> MVIRVLFRPVSLIPVNNSSTPQSQGPISRRLALTALGFGVLAPNVLVACAGKVTKLAEKRPPPAPRLTFRPADSAADVVPIAPISVEVGDGWFQRVALTNSAGKVVAGAYSRDRTIYTITEPLGYDTTYTWSGSAVGHDGKAVPVAGKF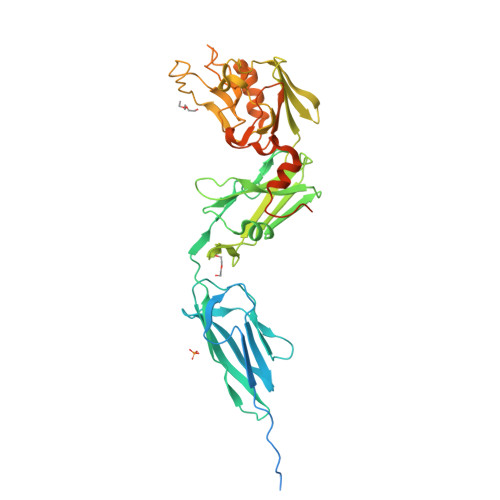TTVAPVKTINAGFQLADGQTVGIAAPVIIQFDSPISDKAAVERALTVTTDPPVEGGWAWLPDEAQGARVHWRPREYYPAGTTVDVDAKLYGLPFGDGAYGAQDMSLHFQIGRRQVVKAEVSSHRIQVVTDAGVIMDFPCSYGEADLARNVTRNGIHVVTEKYSDFYMSNPAAGYSHIHERWAVRISNNGEFIHANPMSAGAQGNSNVTNGCINLSTENAEQYYRSAVYGDPVEVTGSSIQLSYADGDIWDWAVDWDTWVSMSALPPPAAKPAATQIPVTAPVTPSDAPTPSGTPTTTNGPGG>MAMAQELTAMSAWVNQDGSTLYINSINAQGELTGSYINRAAGFACQNSPYPVNGWVFGTAISFSTKWLNSVESCNSITSWSGFYINTGGQGKISTLWQLVVN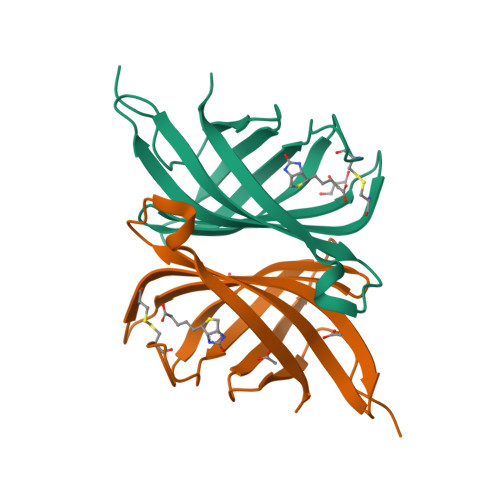GSSSPSQILKGQDVFSQTSA[2x]>SLLNVPAGKDLPEDIYVVIEIPANADPIKYEIDKESGALFVDRFMSTAMFYPCNYGYINHTLSLDGDPVDVLVPTPYPLQPGSVIRCRPVGVLKMTDEAGEDAKLVAVPHSKLSKEYDHIKDVNDLPELLKAQIAHFFEHYKDL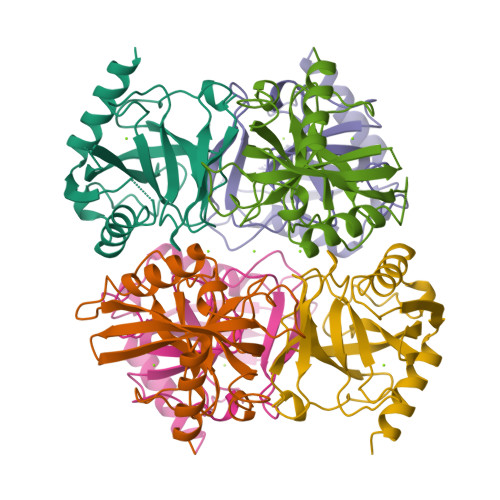EKGKWVKVEGWENAEAAKAEIVASFERAKNK[2x]N6-({[(1S,2E)-cyclooct-2-en-1-yl]oxy}carbonyl)-L-lysine | C15 H26 N2 O4 | 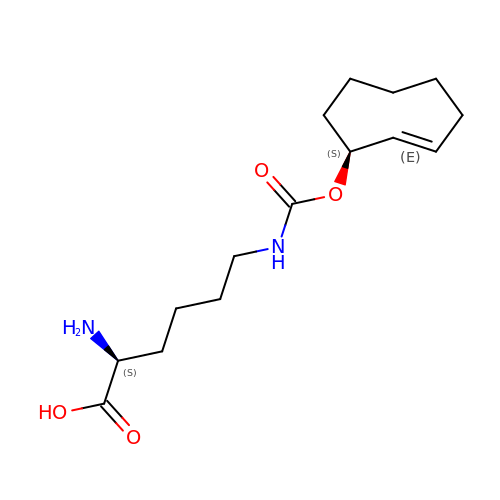RIPRFLAPFPCYBY-OLZOCXBDSA-N>MSDNAQLTGLCDRFRGFYPVVIDVETAGFNAKTDALLEIAAITLKMDEQGWLMPDTTLHFHVEPFVGANLQPEALAFNGIDPNDPDRGAVSEYEALHEIFKVVRKGIKASGCNRAIMVAHNANFDHSFMMAAAERASLKRNPFHPFATFDTAALAGLALGQTVLSKACQ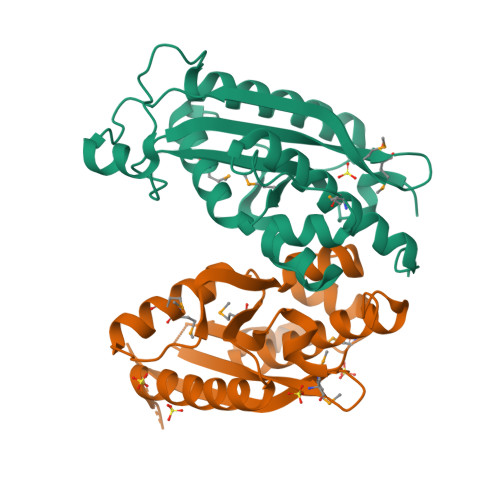TAGMDFDSTQAHSALYDTERTAVLFCEIVNRWKRLGGWPLSAAEEV[4x]> SLMERLGGGGFSARIFVGLNVGDKPTYTIEDVVKDTIAIRKRQGILPDASFVAQRGVYTEQRSGQLVTENSVQIIIIDLEGLSKEDFTGKVQALGKELREDFKQESVIVEIQERGIVQDVYSITAEWYEEGPMRPLRVDLQPSLIS

Svi3-3 represents the first structure of a phage-encoded SAM degrading enzyme. Svi3-3 forms a trimer of ferredoxin-like fold alpha–beta sandwiches, where each subunit has two helices on the outside and a five-stranded anti-parallel beta sheet at the center. The subunits pack in a triangular manner, forming continuous beta sheets with their neighbors and are each in a ‘velcro-like’ topology where residues 2–6 at the N terminus of one subunit form beta-sheet interactions with residues 120–124 in β8 of another subunit. Prompted by DFT calculations producing high energy barriers for a hydrolysis reaction within the active site of Svi3-3, the TLC assays and NMR show unambiguously that Svi3-3 is a SAM lyase forming homoserine lactone and MTA.

When expressed from the T7-promoter expression plasmid, the proteins were highly toxic and the tightly regulated, arabinose-inducible BL21-AI cells had to be used to allow cell growth until induction. An N-terminally truncated 146 amino acid construct of Svi3-3, where the hexahistidine tag had been removed (Svi3-3_d19, Supplementary file 1-table 1), formed crystals in the presence of SAM or the analogue S-adenosyl homocysteine (SAH). The crystals diffracted to 1.45 Å resolution in space group F4132 and the structure was solved using ab initio methods with Arcimboldo (Rodríguez et al., 2009). There is one monomer in the asymmetric unit, forming a trimer around the threefold crystallographic axis. Apart from the disordered C-terminal 16 residues, the full structure could be built. In the structure from co-crystallization with SAM, catalysis has occurred and the product MTA is observed in identical position as the corresponding part of SAH, with the methyl group pointing away from Glu69, while a proline molecule from the cryo buffer is bound in the second half of the active site, mimicking the second product. The protein structures are virtually identical in the presence of SAH and MTA (root mean square deviation [RMSD] of 0.16 Å over 129 Cα atoms). Our activity assay is based on detection of MTA that is also observed in the structure from co-crystallization of Svi3-3 with SAM. Thus, MTA is indeed formed in the reaction. Since MTA and SAH show a perfect overlap between the two structures, any such difference in binding mode between SAM and SAH is likely to involve the methionine end of the substrate, where MD indicates that Tyr58 forms a cation-π interaction with the positively charged sulfur.> MSRKRNRNRSVQVAKATSEQLNVSRMRMSEQGTFALAKVQVDSERMKAEEIRWPHLIGTAESMKQDATVATGLDMLYTFVEKAFKDFKVIPGESEESKKAAKFIEYCLKNMEGQTLRQFARDAATFNEYGLSVVEKVYTQIAVGEYVGKYKVKNLAFRPQASLSRTNPIVYNSDGSAIVGIKQSLSAFQNYTASEIGVGGVSTRMSDVIIPISRVMLMNTGGSSSQALGVSPLVGCYRAWREKILIENLEVVGATKDMGGVIELKIPSQILNKAAMDPSSPEADMVRGLMSDAANAHSGEQSFFMLPSDTKDNAPQYSMTLKGIDG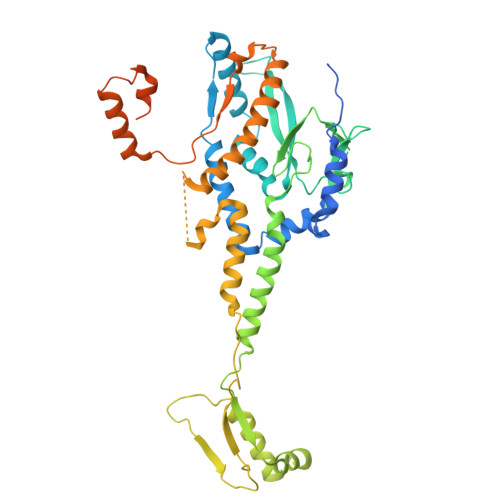MGKQYSTAQLISDRKKSILDRLGAGFINVGNDKGGSYNLSESKQTIHTQFVQRVNEIILEALNENLLPQLLALNDIRLPETEMPYVKAGEIVDVDMEGFSKAIQRIGAVGYLPKTPKVINRVLEVLGIDEKIEEDISQEELMKLLGEDTSRAGDGMTKGSSGNGTGKISASRDNSAANLDN>MTGNAKLIDRVSAINWNRLQDEKDAEVWDRLTGNFWLPEKVPVSNDIPSWGTLTAGEKQLTMRVFTGLTMLDTIQGTVGAVSLIPDALTPHEEAVLTNIAFMESVHAKSYSQIFSTLCSTAEIDDAFRWSEENRNLQRKAEIVLQSYRGDEPLKRKVASTLLESFLFYSGFYLPMYWSSRAKLTNTADMIRLIIRDEAVHGYYIGYKFQRGLALVDDVTRAELKDYTYELLFELYDNEVEYTQDLYDEVGLTEDVKKFLRYNANKALMN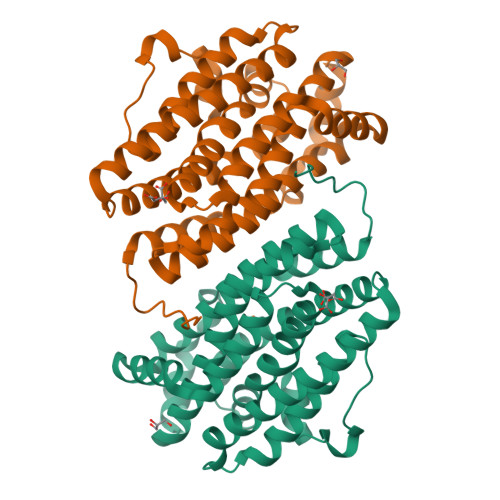LGYEALFPRDETDVNPAILSALSPNAD[3x]In general, type IIa bacteriocins are coexpressed with cognate immunity proteins (pediocin-like immunity proteins) composed of 88~115 amino acids, in order to protect the organism from the antimicrobial activity of its own bacteriocin. Based on the remarkable degree of sequence identity (~99%) of PedB of P. pentosaceus to that of P. acidilactici, we regarded PedB as the immunity protein against pediocin PP-1. PedB is a small positively charged protein with 112 amino acids and belongs to subgroup A. No transmembrane helices are predicted from sequence analysis. The 1.6 Å crystal structure of PedB reveals that PedB consists of an antiparallel four-helix bundle with a flexible C-terminal end.

The initial model was built according to the phased electron density map obtained by using anomalous scattering differences of selenium atoms in the selenomethionyl L24M crystal. A final model for native PedB was refined subsequently to 1.6 Å resolution against native data. The native PedB crystals contain one molecule in the asymmetric unit. Out of the total 112 amino acids in native PedB, residues 7–93 are visible in the crystal structure. The crystal structure reveals that PedB forms a compact globular domain composed of four helices. They are arranged so that α1 and α3 run in the same direction and α2 and α4 in the opposite direction, forming an antiparallel four-helix bundle. The relative disposition of the four helices of PedB is maintained mainly by a network of hydrophobic interactions in the core of the molecule: Phe17, Leu20, and Leu24 from α1 (residues 9–26), Leu48 from α2 (residues 31–49), Val61 and Ile65 from α3 (residues 55–72), Leu74 and Phe76 from the loop between α3 and α4, Leu84 and Ile87 from α4 (residues 80–92) form a hydrophobic core. The C-terminal end of PedB (residues 94–112) that is thought to be important for immunity has no electron density, suggesting that this region is flexible. As expected, the structure of PedB is well-superimposed to that of EntA-im with r.m.s.d. of 1.3 Å for all Cα atoms. Deletion of last four residues (PedB1–108) resulted in severe loss of immunity compared to the wild type PedB, and deletion of seven residues (PedB1–105) almost completely abolished the activity.

> MNKTKSEHIKQQALDLFTRLQFLLQKHDTIEPYQYVLDILETGISKTKHNQQTPERQARVVYNKIASQALVDKLHFTAEENKVLAAINELAHSQKGWGEFNMLDTTNTWPSQ>GMKVTNYQGATIDPYSKGLGMVPGTSIQLTDAARLEWNLLNEDVSLPAAVLYADRVEHNLKWMQAFVAEYGVKLAPHGKTTMAPQLFRRQLETGAWGITLATAHQVRAAYHGGVSRVLMANQLVGRRNMMMVAELLSDPEFEFFCLVDSVEGVEQLGEFFKSVNKQLQVLLELGVPGGRTGVRDAAQRNAVLEAITRYPDTLKLAGVELYEGVLKEEHEVREFLQSAVAVTRELVEQERFARAPAVLSGAGSAWYDVVAEEFVKASETGKVEVVLRPGCYLTHDVGIYRKAQTDIFARNPVAKKMGEGLLPALQLWAYVQS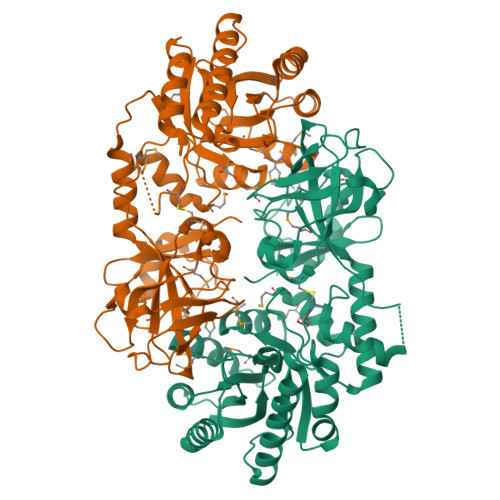IPEPDRAIIGLGKRDSAFDAGMPEPARHYRPGNEAPRDIAASEGWEIFGLMDQHAYLRIPAGADLKVGDMIAFDISHPCLTFDKWRQVLVVDPAYRVTEVIETFF[2x]The V. cholerae T4aP secretin PilQ is a member of the bacterial secretin superfamily. Bacterial secretins are united by a common C-terminal secretin domain, which oligomerizes to form a large pore in the outer membrane. During natural transformation, the T4aP extends and retracts a filament to take up DNA cargo. The T4aP machinery extends and retracts the T4aP through the PilQ outer membrane pore.

Here, we present the structure of the V. cholerae T4aP secretin PilQ to ~2.7 Å using a fully functional, His-tagged allele that we express and purify from the native bacterium. The cryoEM structure (C14 symmetry, overall resolution of 2.7 Å at Fourier shell correlation (FSC) of 0.143, and 3 Å at FSC of 0.5) reached sufficient, isotropic resolution to recognize and model residues 160–571 of VcPilQ, which includes the N0, N3, and secretin domains. Once assembled, VcPilQ forms a 56-strand beta barrel. Inside the barrel, two further beta hairpins (beta strand-turn-beta strand each) form a gate. In VcPilQ, a 32 Å alpha helix follows the N0 domain. Following the end of this helix, the protein chain changes direction (~104° angle) as the coil flows into the N3 domain. This dramatically reduces the channel diameter, from 90 Å at the bottom of the N0 domain to 60 Å across the N3 domain. The inner beta lip, N3, and coil regions of VcPilQ are all negatively charged. In our VcPilQ atomic model, the distances between the bottom of the AHL to the top of the beta strands is about 3 nm, which is substantially taller than the same region in the previously published T2SS structures. In our VcPilQ structure, the inner channel distance between the corresponding glycine (G439) alpha carbons is about 8 nm.

>[14x]MRNGLKTYVAQTWLTLWVGLALCASSTVFSAEFATTNQLENIDFRVNKEKAAVLIVELASPSAVVDVQKVQEGLNIELLKTDVADDKLYLLDVKDFSTPVESVEVFRKAPSTQLVVTVDGEFQHDYTLKGKYLEVVISKLKADEKPKPKSVLEKEGKLISINFQDIPVRNVLQLIADYNGFNLVVSDSVVGNLTLRLDGVPWQQVLDIILQVKGLDKRVDGNVILIAPKEELDLREKQALEKARLAEELGDLKSEIIKINFAKASDIAAMIGGEGNVNMLSERGSISIDERTNSLLIRELPDNIAVIREIIESLDIPVKQVQIEARIVTVKEGNLEELGVRWGVMSTNGSHSVGGSIESNLWQKGLLADDEFPVDEFLNVNLASTSANASSIAFQVAKLGSGTLLDLELSALQNESKAEIISSPRLITTNKQPAYIEQGTEIPYLESSSSGASTVAFKKAVLSLKVTPQITPDNRLVLDLSVTQDRRGETVKTGTGEAVSIDTQRIGTQVLVNNGETVVLGGIFQHSINNSVDKVPLLGDLPVLGALFRRTYEQMGKSELLIFVTPKVVIQ>APITAPDITSICKDASSGIGNQEGAIRTRKCCPPSLGKKIKDFQFPNDKKVRMRWPAHKGTKKQVDDYRRAIAAMRALPDDDPRSFVSQAKIHCAYCNGGYTQVDSGFPDIDIQIHNSWLFFPFHRWYLYFYERILGSLIDEPNFALPYWKWDEPKG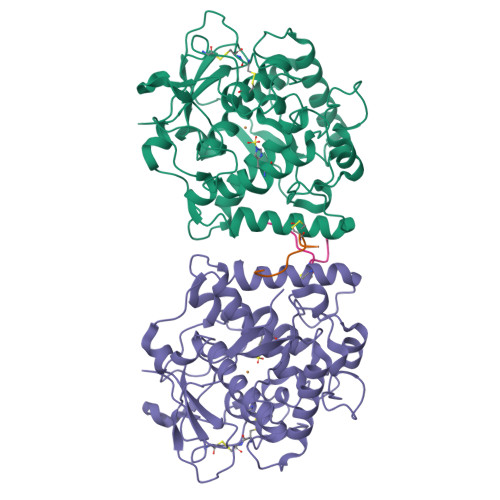MPISNIFLGDASNPLYDQYRDANHIEDRIVDLDYDGKDKDIPDQQQVACNLSTVYRDLVRNGVDPTSFFGGKYVAGDSPVANGDPSVGSVEAGSHTAVHRWVGDPTQPNNEDMGNFYSAGYDPVFYIHHANVDRMWKLWKELRLPGHVDITDPDWLNASYVFYDENKDLVRVYNKDCVNLDKLKYNFIENSKE[4x];>DGVFTTPCDPEYAGG[4x]> SMTKAAAPGVEDEPLLRENPRRFVIFPIEYHDIWQMYKKAEASFWTAEEVDLSKDIQHWESLKPEERYFISHVLAFFAASDGIVNENLVERFSQEVQITEARCFYGFQIAMENIHSEMYSLLIDTYIKDPKEREFLFNAIETMPCVKKKADWALRWIGDKEATYGERVVAFAAVEGIFFSGSFASIFWLKKRGPMPGLTFSNELISRDEGLHC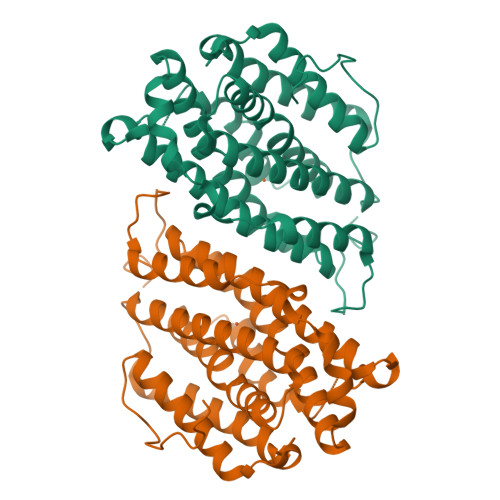DFACLMFKHLVHKPSEERVREIIINAVRIEQEFLTEALPVKLIGMNCTLMKQYIEFVADRLMLELGFSKVFRVENPFDFMENISLEGKTNFFEKRVGEYQRMGVMSSPTENSFTLDADF> MSHSSAPER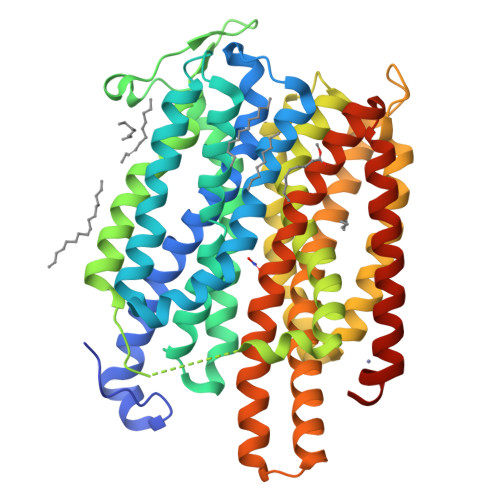ATGAVITDWRPEDPAFWQQRGQRIASRNLWISVPCLLLAFCVWMLFSAVAVNLPKVGFNFTTDQLFMLTALPSVSGALLRVPYSFMVPIFGGRRWTAFSTGILIIPCVWLGFAVQDTSTPYSVFIIISLLCGFAGANFASSMANISFFFPKQKQGGALGLNGGLGNMGVSVMQLVAPLVVSLSIFAVFGSQGVKQPDGTELYLANASWIWVPFLAIFTIAAWFGMNDLATSKASIKEQLPVLKRGHLWIMSLLYLATFGSFIGFSAGFAMLSKTQFPDVQILQYAFFGPFIGALARSAGGALSDRLGGTRVTLVNFILMAIFSGLLFLTLPTDGQGGSFMAFFAVFLALFLTAGLGSGSTFQMISVIFRKLTMDRVKAEGGSDERAMREAATDTAAALGFISAIGAIGGFFIPKAFGSSLALTGSPVGAMKVFLIFYIACVVITWAVYGRHSKKLESSGENLYFQG Three MICAL isoforms (MICAL-1, -2, and -3) have been identified in vertebrates. RP/EBs5 as well as MICALs contain a single type-2 CH domain. F-actin, leading to destabilization and disruption of actin filaments. the oxidation of Met 44 of actin by MICAL.

of the structure of a MICAL fragment containing the entire MO and CH domains. 0.25 and 0.30 using data to 2.31 Å resolution. one single chain monomer per asymmetric unit. used for crystallization MICALMO-CH is a monomer in solution. domain and residues 506–554 and 562–614 of the CH domain. the 19-residue linker that connects the MO and CH domains. is compatible with a flexible linker between the two domains. greater for MICALMO-CH than that for the isolated MO domain. MICALMO-CH, is found in the kinetics of oxidation of actin. significantly increase the efficiency of actin modification by MICAL.

> GASPASTNPAHDHFETFVQAQLCQDVLSSFQGLCRALGVESGGGLSQYHKIKAQLNYWSAKSLWAKLDKRASQPVYQQGQACTNTKCLVVGAGPCGLRAAVELALLGARVVLVEKRIKFSRHNVLHLWPFTIHDLRALGAKKFYGRFCTGTLDHISIRQLQLLLLKVALLLGVEIHWGVKFTGLQPPPRKGSGWRAQLQPNPPAQLASYEFDVLISAAGGKFVPEGFTIREMRGKLAIGITANFVNGRTVEETQVPEISGVARIYNQKFFQSLLKATGIDLENIVYYKDETHYFVMTAKKQCLLRLGVLRQDLSETDQLLGKANVVPEALQRFARAAADFATHGKLGKLEFAQDARGRPDVAAFDFTSMMRAESSARVQEKHGARLLLGLVGDCLVEPFWPLGTGVARGFLAAFDAAWMVKRWAEGAGPLEVLAERESLYQLLSQTSPENMHRNVAQYGLDPATRYPNLNLRAVTPNQVQDLYDMMDKEHAQRKSDEPDSRKTTTGSAGTEELLHWCQEQTAGFPGVHVTDFSSSWADGLALCALVHHLQPGLLEPSELQGMGALEATTWALRVAEHELGITPVLSAQAVMAGSDPLGLIAYLSHFHSAFKNTSH>LKESPSGYLRSGEGDTGCGELVWVGEPVTLRTAETITGKYGVWMRDPKPVYPYTQETTWRIDTVGTDVRQVFEYDLISQFMQGYPSKVHILPRPLESTGAVVYNGSLYFQGAGSRTVIRYDLKTETVKAEKEIPGAGYHGQYPYSWGGYTDIDLAVDENGLWVIYSTNQAKGNIVLSKLNPETLEVEQTWETNIRKQ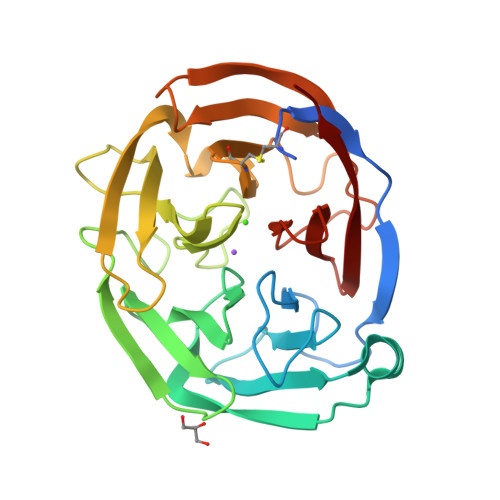SVANAFIICGTLYTVSSYTSADATVNFAYDTNTGTSKYLDIPFKNRYKYNSMIDYNPLERKLFAWDNGHMVTYDIKLSKM[2x]> MPARRPFIGGNFKCNGSLDFIKSHVAAIAAHKIPDSVDVVIAPSAVHLSTAIAANTSKQLRIAAQNVYLEGNGAWTGETSVEMLQDMGLKHVIVGHSERRRIMGETDEQSAKKAKRALEKGMTVIFCVGETLDERKANRTMEVNIAQLEALGKELGESKMLWKEVVIAYEPVWSIGTGVVATPEQAEEVHVGLRKWFAEKVAAEGAQHIRIIYGGSANGSNCEKLGQCPNIDGFLVGGA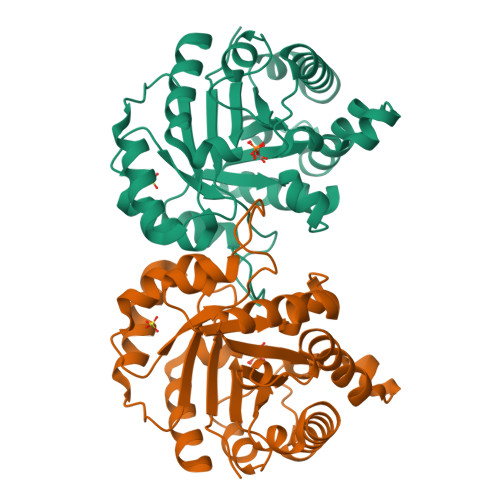SLKPEFMTMIDILTKTRT> MPKVIENVGCPYCGCSCDDVRITVSDDGKDILEVENVCAIGTEIFKHGCSKDRIRLPRMRQPDGSMKDISYEEAIDWTARHLLKAKKPLMYGFGSTNCEGQAAAARVMEIAGGMLDNC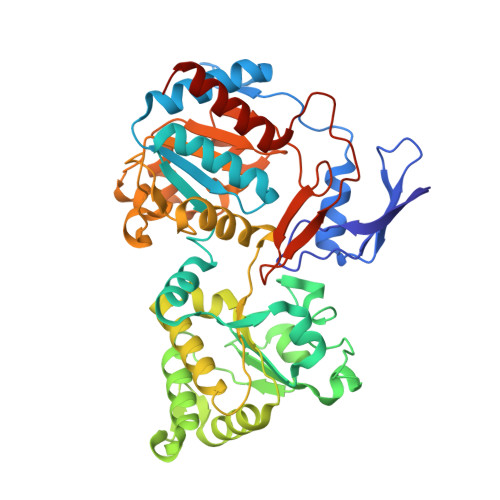ATICHGPSFLAIFDNGYPSCTLGEVKNRADVIVYWGSNPAHAHPRHMSRYSIFPRGFFTGKGQKKRTVIVIDPRFTDTANVADYHLQVKQGHDYELFNAFRMVIHGHGKDLPDEVAGIKKETILEVAEIMKNARFGTTFFGMGLTHTDGRNHNIDIAISLTRDLNKISKWTIMAMRGHYNIAGPGVVWSWTFGFPYCLDLTKQNHAHMNPGETSSVDMAMRDEVDMFINIGTDAAAHFPIPAVKQLKKHPWVTIDPSINMASEISDLHIPVCICGVDVGGIVYRMDNVPIQFRKVIEPPEGVMDDETLLNKIADRMEELKAKGEA4-[5-[(4~{a}~{R},8~{a}~{S})-4-oxidanylidene-3-propan-2-yl-4~{a},5,8,8~{a}-tetrahydrophthalazin-1-yl]-2-methoxy-phenyl]-~{N}-(2-azanyl-2-oxidanylidene-ethyl)benzamide 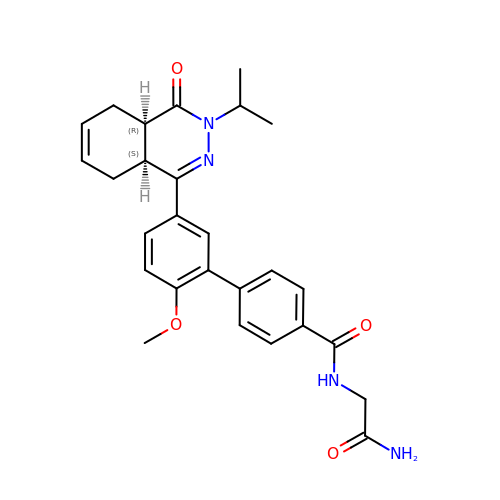| C27 H30 N4 O4 | STNWAGAHKRPYDJ-LEWJYISDSA-N>[6x]ALKRKIEAAKMPKDAREKTEAELQKLKMMSPMSAEATVVRGYIDWMLQVPWNSRSKVKKDLVKAQEVLDTDHYGLERVKDRILEYLAVQSRVSKIKGPILCLVGPPGVGKTSLGQSIAKATGRQYVRMALGGVRDEAEIRGHRRTYIGSMPGKLIQKMAKVGVKNPLFLLDEIDKMASDMRGDPASALLEVLDPEQNVAFNDHYLEVDYDLSDVMFVATSNSMNIPAPLLDRMEVIRLSGYTEDEKLNIAKQHLLPKQFERNAIKKGELTIDDSAIMSIIRYYTREAGVRSLEREISKLCRKAVKNLLMDKTVKHIEINGDNLKDFLGVQKVDYGRADTENRVGQVTGLAWTEVGGDLLTIETACVPGKGKLTYTGSLGEVMQESIQAALTVVRARADKLGINPDFYEKRDIHVHVPEGATPKDGPSAGIAM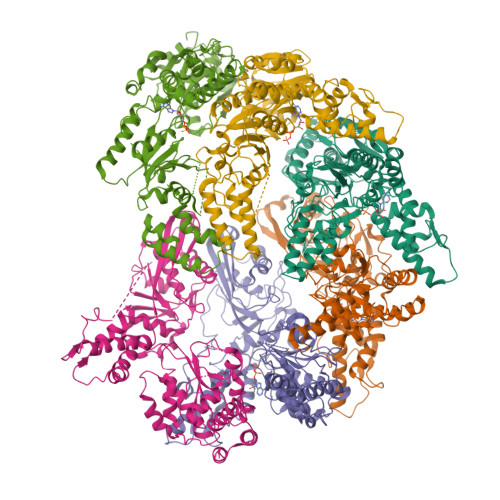CTALVSCLTGNPVRADVAMTGEITLRGLVLPIGGLKEKLLAAHRGGIKVVLIPDDNKRDLEEIPDNVIADLEIHPVKRIDDVLAIALEHPA> ASWIKEGELSLWERFCANIIKAGPMPKHIAFIMDGNRRYAKKCQVERQEGHSQGFNKLAETLRWCLNLGILEVTVYAFSIENFKRSKSEVDGLMDLARQKFSRLMEEKEKLQKHGVCIRVLGDLHLLPLDLQELIAQAVQATKNYNKCFLNVCFAYTSRHEISNAVREMAWGVEQGLLDPSDISESLLDKCLYTNRSPHPDILIRTSGEVRLSDFLLWQTSHSCLVFQPVLWPEYTFWNLFEAILQFQMNHSMLQKARDMYAEERKRQQLERDQATVTEQLLREGLQASGDAQLRRTRLHKLSARREERVQGFLQALELKRADWLARLGT;> AAHHRMRWRADGRSLEKLPVHMGLVITEVEQEPSFSDIASLVVWCMAVGISYISVYDHQGIFKRNNSRLMDEILKQQQELLGLDCSKYSPEFANSNDKDDQVLNCHLAVKVLSPEDGKADIVRA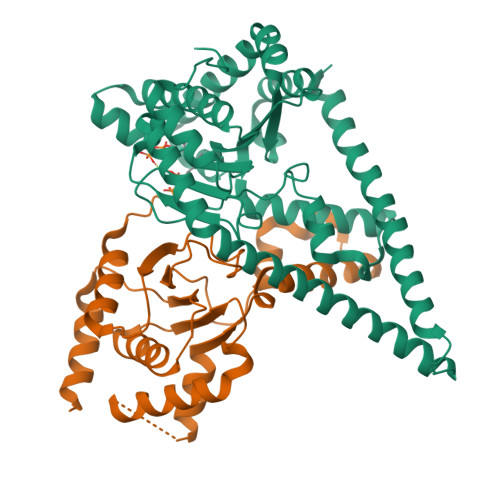AQDFCQLVAQKQKRPTDLDVDTLASLLSSNGCPDPDLVLKFGPVDSTLGFLPWHIRLTEIVSLPSHLNISYEDFFSALRQYAACEQRLGK> MALFGSNDVTTAHSDYEIVLEGGSSSWGKVKARAKVNAPPASPLLPADCDVKLNVKPLDPAKGFVRISAVFESIVDSTKNKLTIEADIANE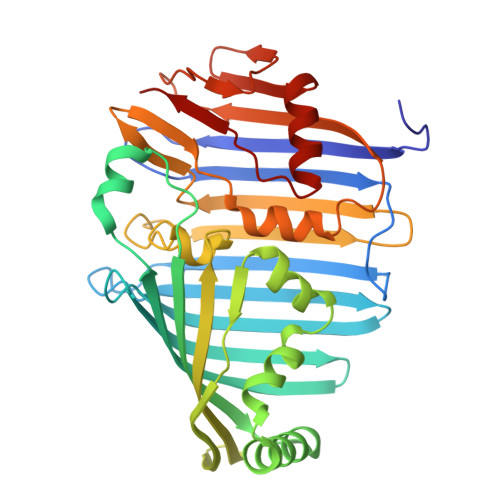TKERRISVGEGMVSVGDFSHTFSFEGSVVNLFYYRSDAVRRNVPNPIYMQGRQFHDILMKVPLDNNDLIDTWEGTVKAIGSTGAFNDWIRDFWFIGPAFTALNEGGQRISRIEVNGLNTESGPKGPVGVSRWRFSHGGSGMVDSISRWAELFPSDKLNRPAQVEAGFRSDSQGIEVKVDGEFPGVSVDAGGGLRRILNHPLIPLVHHGMVGKFNNFNVDAQLKVVLPKGYKIRYAAPQYRSQNLEEYRWSGGAYARWVEHVCKGGVGQFEILYAQ>SNAMNR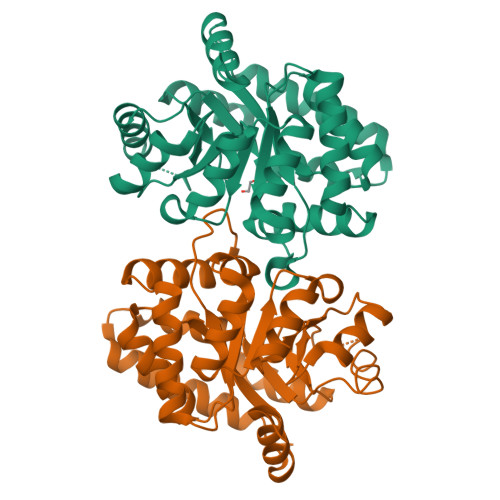YQALFQRLSAAQQGAFVPFVTIGDPNPEQSLAIMQTLIDAGADALELGMPFSDPLADGPTIQGANLRALAAKTTPDICFELIAQIRARNPETPIGLLMYANLVYARGIDDFYQRCQKAGVDSVLIADVPTNESQPFVAAAEKFGIQPIFIAPPTASDETLRAVAQLGKGYTYLLSRAGVTGAETKANMPVHALLERLQQFDAPPALLGFGISEPAQVKQAIEAGAAGAISGSAVVKIIETHLDNPAKQLTELANFTQAMKKATKI[2x]> MGHHHHHHHHHHSSGHIDDDDKHMAGGAAQESKSFAVGMFKGQLTTDQVFPYPSVLNEEQTQFLKELVEPVSRFFEEVNDPAKNDALEMVEETTWQGLKELGAFGLQVPSELGGVGLCNTQYARLVEIVGMHDLGVGITLGAHQSIGFKGILLFGTKAQKEKYLPKLASGETVAAFCLTEPSSGSDAASIRTSAVPSPCGKYYTLNGSKLWISNGGLADIFTVFAKTPVTDPATGAVKEKITAFVVERGFGGITHGPPEKKMGIKASNTAEVFFDGVRVPSENVLGEVGSGFKVAMHILNNGRFGMAAALAGTMRGIIAKAVDHATNRTQFGEKIHNFGLIQEKLARMVMLQYVTESMAYMVSANMDQGATDFQIEAAISKIFGSEAAWKVTDECIQIMGGMGFMKEPGVERVLRDLRIFRIFEGTNDILRLFVALQGCMDKGKELSGLGSALKNPFGNAGLLLGEAGKQLRRRAGLGSGLSLSGLVHPELSRSGELAVRALEQFATVVEAKLIKHKKGIVNEQFLLQRLADGAIDLYAMVVVLSRASRSLSEGHPTAQHEKMLCDTWCIEAAARIREGMAALQSDPWQQELYRNFKSISKALVERGGVVTSNPLGF

Very long-chain acyl-CoA dehydrogenase (VLCAD) is an inner mitochondrial membrane enzyme that catalyzes the first and rate-limiting step of long-chain fatty acid oxidation. Whereas SCAD, MCAD, and LCAD operate as tetramers in the mitochondrial matrix and share considerable sequence homology, VLCAD is an outlier that localizes to the inner mitochondrial membrane as a dimer and contains a unique additional stretch of 180 amino acids at its C-terminus. The unique C-terminal region is comprised of an α-helical bundle that lies perpendicular to the enzyme and further includes a non-visualized region spanning amino acids 446–478 believed to mediate membrane interaction. Point mutations in human VLCAD can produce an inborn error of metabolism called VLCAD deficiency that can lead to severe pathophysiologic consequences, including cardiomyopathy, hypoglycemia, and rhabdomyolysis.

Specifically, on the N-terminal side of the density gap, the structure demonstrated residues through amino acid 459 facing away from the protein, consistent with a module capable of projecting outward to engage a membrane surface. No secondary structure was evident in this region and residues 460–475 remain unresolved, and thus highly flexible, in this structure generated in the solution phase. Of note, the crystal contacts demonstrated a reciprocal interaction between the outwardly projecting MBR of one VLCAD dimer and the surface groove of its neighboring dimer, consistent with a stabilizing interaction for this otherwise exposed and disordered region. The HDX MS profile of VLCAD in solution, evaluated after 10 s, 1 m, 10 m, and 1 h of deuteration, was consistent with the structural organization seen by X-ray crystallography, including general agreement between deuteration and crystallographic B factors. In contrast, the various mainly structured regions, including the α-helical domain 1 (aa 56–165), β-sheet domain (aa 166–276), α-helical domain 2 (aa 277–445), and α-helical domain 3 (aa 479–615), exhibited an overall low level of deuterium uptake that only modestly increased in a time-dependent fashion. Notably, that portion of the C-terminus containing the MBR and not fully resolved by X-ray crystallography (e.g., aa 446–478) displayed a high degree of deuterium uptake from early to late labeling times, consistent with marked flexibility of this region in solution. Taken together, the X-ray crystallography, HDX MS, and liposomal translocation assays indicate that, in solution, the structurally-unresolved portion of the C-terminal region is solvent-exposed, conformationally dynamic, and essential to VLCAD interaction with cardiolipin-enriched membrane. Interestingly, the structurally unresolved portion of the C-terminal region (e.g., aa 446–478) is predicted to fold as a helix-turn-helix hairpin based on sequence homology to structured proteins in the database.>[2x]AETVESCLAKPHTENSFTNVWKDDKTLDRYANYEGCLWNATGVVVCTGDETQCYGTWVPIGLAI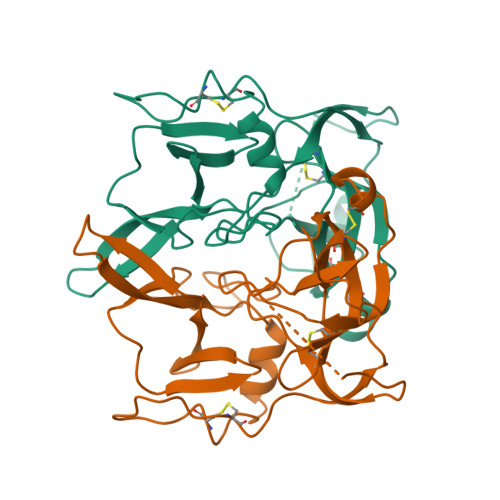PENEGGGSEGGGSEGGGSEGGGTKPPEYGDTPIPGYTYINPLDGTYPPGTEQNPANPNPSLEESQPLNTFMFQNNRFRNRQGALTVYTGTVTQGTDPVKTYYQYTPVSSKAMYDAYWNGKFRDCAFHSGFNEDPFVCEYQGQSSDLPQPPVNAAAHHHHHH> MLRRTSRRLLGYTPINPDTSPMLMYSQCHWHYNLPQGMERPSSVNRSLPAPYQPHHSSVNKYRGVWISTEMHPAFLVGLAPQLKKLPHGRVVPQTPVAEVIDEFNKLSPLIDDAAARDGWLAKIFQHCAFQRSGAEAMALWDKHCAPRFMRDDSASAPPLPLVQAILFCCSKSDSAEWRPIFTKCLKDGWNYTPSFDTPQWSYLLKSLGRQGDEEGVRLVLEEMADVQADLDRVEARSLVYALNAVHDKAIYNYVKKYLFYLGERKVKFLRITYADLRGHGAEKLRVPLKENDSMFYHVCWHASIRQPRQFSPRQLYFDYAPSQLATSGHSPNAKVDGIVKDKIDKWKAEGLLPEDYVHEDRVYDRTAAFKSVARQEKWKKVPRIVKSKR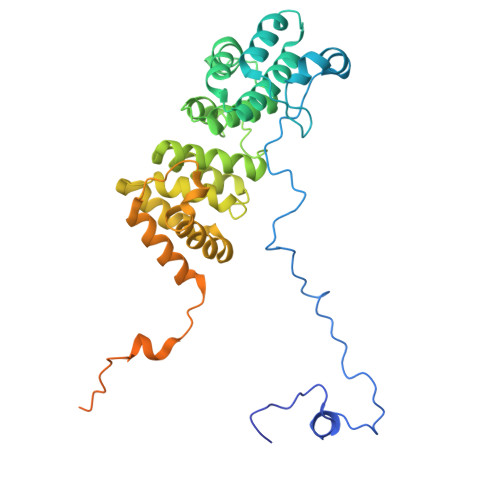FGYSGEP> MLIRRLRRPHSTVRGCRISSASNSDSAGAFSANGTQLPDPPYYLPHSPRFDAERCGTFNKKWLLNLPALKPLVRNSTYLPKKEELWRAPTHEALETIIGHLPYHDALRYITEHSLFLLFPTV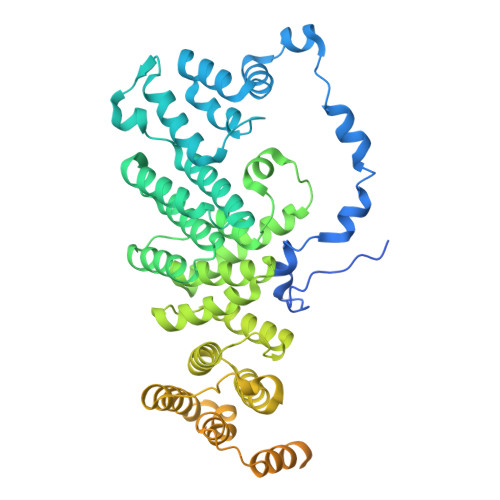LRARDAPLPHVIYEDFMKSCTFASLQNPPEEQFALPSVLLRTLLCMAAYHCTLDADYFTTCQMLFGRMEQQQQTTPEVLSAWVYCCTASGRVDEALTYAKYMADCSAPFDVTVFSLMQHPSLNPIEVEDGSVPHSAKGLLLQRRLGNRLHTAYRSDAVAAHGMFVYYALTLSHVRKWEVIRAAAALGVTLAERTVVLAVEVFAREKGMRCGPKTVKALTHFLAQDGTVGHLLYVLLRARKNELLPEFRDLPHTTFSEEEQELVLQCVAQRARHDDSFAVAATLVSSLVREDDPSELLMAFARAARNHHSADVCGGDGDGSVCADVPAPVPESPPSNSSEIIEKDRWAVVQASVRSLLLDVNALDQASRRDAYHKHWKNGNKGVKNKENVLAKTLTLPHDSMHTATIQRKEKELWELMRSDTPVGVRELAQLNIMEELQEAKRLERAEMAWVNPDGTF2-(9-chloro-1H-phenanthro[9,10-d]imidazol-2-yl)benzene-1,3-dicarbonitrile | 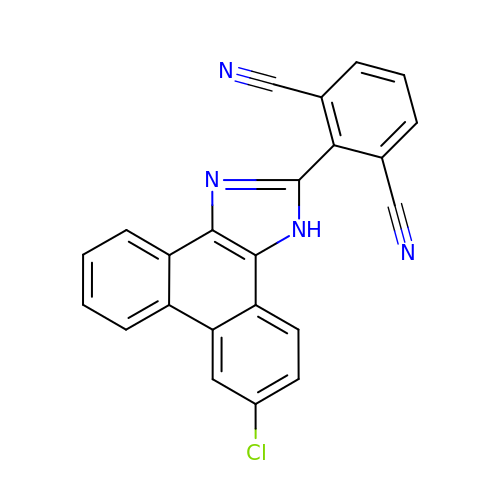C23 H11 Cl N4 | BVFLHOOKHPFDCT-UHFFFAOYSA-N> MAKPIADDIVVRQVDVGETEQLMTFLLAHYYPEEPLTAGTHPPEPEAADKEFLLSNVPFGTCFVALHEGRIVAAVVAGPKDSHEPEHMAEEARKYAGGKWGSILHLLSAVETATDV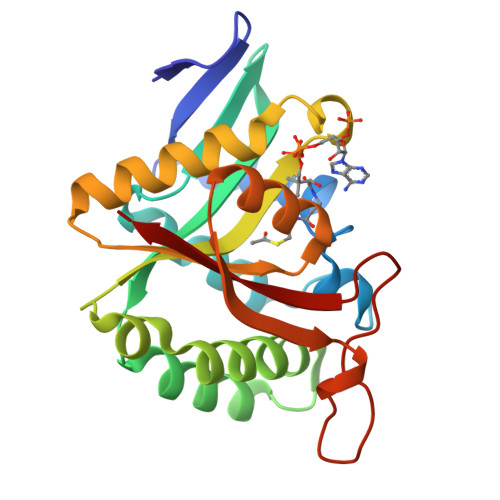CRRFSVPSCLHVHALGVDPQLRGRNLGGRLMETVAQRGRDLGHQLVSVDCTSVYAARLVQRLGYQLINTLRYVDHLDASGQQVIRPPPPHESVQTFVLHL>[4x]GNGKLRQWLIDQIDSGKYPGLVWENEEKSIFRIPWKH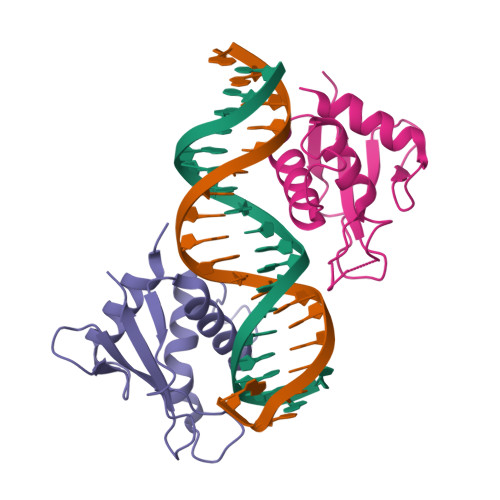AGKQDYNREEDAALFKAWALFKGKFREGIDKPDPPTWKRRLRCALNKSNDFEELVERSQLDISDPYKVYRIVPEGAKKG agropinic acid | C11 H17 N O8 | 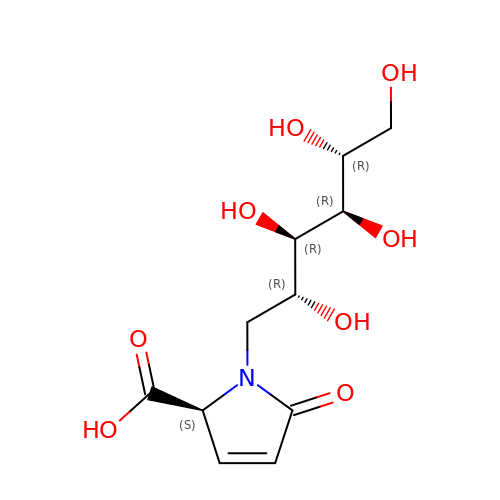WYIHPABVKQQJFB-SZWOQXJISA-N>[2x]MNNNFQDNQTINLIQSRRSIRKFTTEQISDEQVNTLLHCAFAAPSGCNKQPWHITVVQDQKLLKEISDDTLSRIHEVSN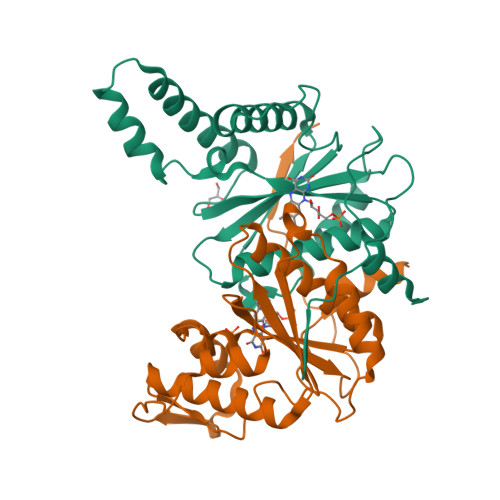VEINKNFKLFYGAPTVLFISYDESSSWAPYDIGILTGNITTAAQALGLGSCIIGMVRGLFTPVEQGDIEGLVSVLDKEDVKESESIKMKFDTNKKYRELLDIPEGYSVPFGIAVGIPDGNLPNAREVVYKVSRVAENLYFQGHHHHHHHHHH>XHLTIHTWPEYGYAAIDLFTCGEDVDPWKAFEHLKKALKAKRVHVVEHERGRYDEIGIPEDSPHKAAV[2x];>MKSLGRHLVAEFYECDREVLDNVQLIEQEMKQAAYESGATIVTSTFHRFLPYGVSGVVV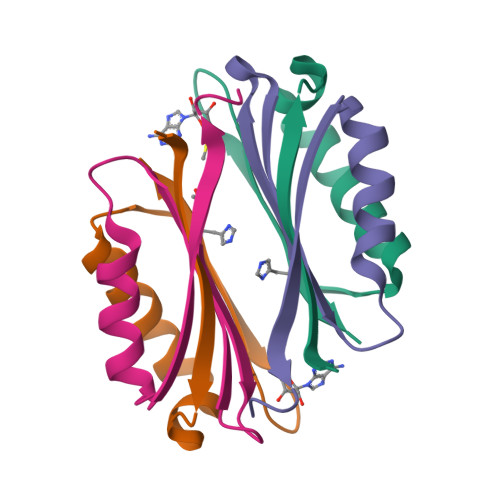ISE[2x]>MGSDKIHHHHHHENLYFQGMKIALIIENSQAAKNAVVHEALTTVAEPLGHKVFNYGMYTAEDKASLTYVMNGLLAGILLNSGAADFVVTGCGTGMGSMLAANAMPGVFCGLVIDPTDAFLFGQINDGNAISMPYSKGFGWAAELNLQDVYRKLFDGERGLGYPRERAEIMRKNRG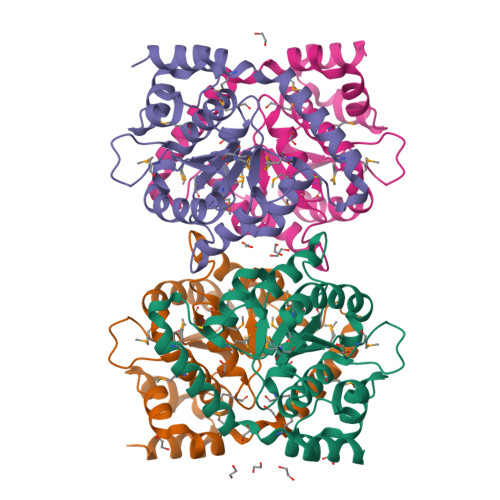ILRELKDASCRDMLTVLKTVDQDLLRAAIAGEKFAELFYPNCKDDAIANYLRSLDA[16x]{(1r,4r)-4-[4-(4-amino-7,7-dimethyl-7H-pyrimido[4,5-b][1,4]oxazin-6-yl)phenyl]cyclohexyl}acetic 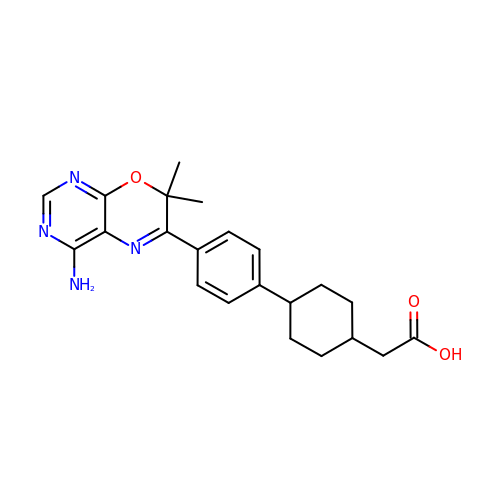acid | C22 H26 N4 O3 | FUIYMYNYUHVDPT-HDJSIYSDSA-N>GPGSMAPTQLEQCASHGKLLQEKKKLEKLHLRDLLKDEARNDLLIRSTDQGVYLDFSRQKITLETLQHLVNLAHERQVPAMVKRMFSGEKINQTENRAVLHVALRMPEGSEPVHVDGKNVLDEVHAVLRRIRVFSEKVRSGEIRGHTGKKLVNVISIGIGGSYLGTEFVHLALAAEGYAAEKAHGRQIHFLANVDPVDVWLAERGFDPEETLVVVISKTFTTAETMMNARSVRDWYLHHYKGDERALGAHFCAVSTNLDGTSKFGIQSDRVFGFWDWVGGRYSVTSAVGILPLALQYGYDVAQEFLNGAHAMDVHFKTAELADNLPMLMGLISVWNATFFGYSNVAVLPYAQALLRFPAHIQQLTMESNGKRVTMDGKTLDFDVGEIFFGEPGTNGQHSFYQLIHQGRVIPAEFIGFCKSQRAIKLKEEPVS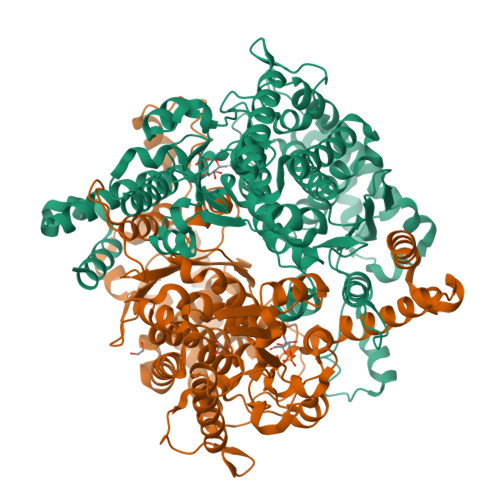NHDELMSNFFAQPDALAFGKTPEELRKEGIPEKLVPHKTFPGDRPSCMLLFPEISPFHIGQLLALYEHRVAVEGWLWGINSFDQWGVELGKVLAKGVRGILQKRREGKAPHESGQSELCSSTRKILEHYVQQSKA[2x]> NQSVVVDFLLPTGVYLNFPVSRNANLSTIKQLLWHRAQYEPLFHMLSGPEAYVFTCINQTAEQQELEDEQRRLCDVQPFLPVLRLVAREGDRVKKLINSQISLLIGKGLHEFDSLCDPEVNDFRAKMCQFCEEAAARRQQLGWEAWLQYSFPLQLEPSAQTWGPGTLRLPNRALLVNVKFEGSEESFTFQVSTKDVPLALMACALRKKATVFRQPLVEQPEDYTLQVNGRHEYLYGSYPLCQFQYICSCLHSGLTPHLTMVHSSSILAMRDEQSNPAPQVQKPRAKPPPIPAKKPSSVSLWSLEQPFRIELIQGSKVNADERMKLVVQAGLFHGNEMLCKTVSSSEVSVCSEPVWKQRLEFDINICDLPRMARLCFALYAVIEKAKKARSTKKKSKKADCPIAWANLMLFDYKDQLKTGERCLYMWPSVPDEKGELLNPTGTVRSNPNTDSAAALLICLPEVAPHPVYYPALEKILELGRHSECVHVTEEEQLQLREILERRGSGELYEHEKDLVWKLRHEVQEHFPEALARLLLVTKWNKHEDVAQMLYLLCSWPELPVLSALELLDFSFPDCHVGSFAIKSLRKLTDDELFQYLLQLVQVLKYESYLDCELTKFLLDRALANRKIGHFLFWHLRSEMHVPSVALRFGLILEAYCRGSTHHMKVLMKQGEALSKLKALNDFVKLSSQKTPKPQTKELMHLCMRQEAYLEALSHLQSPLDPSTLLAEVCVEQCTFMDSKMKPLWIMYSNEEAGSGGSVGIIFKNGDDLRQDMLTLQMIQLMDVLWKQEGLDLRMTPYGCLPTGDRTGLIEVVLRSDTIANIQLNKSNMAATAAFNKDALLNWLKSKNPGEALDRAIEEFTLSCAGYCVATYVLGIGDRHSDNIMIRESGQLFHIDFGHFLGNFKTKFGINRERVPFILTYDFVHVIQQGKTNNSEKFER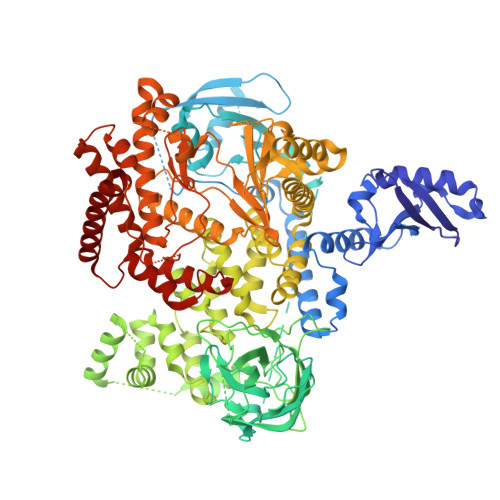FRGYCERAYTILRRHGLLFLHLFALMRAAGLPELSCSKDIQYLKDSLALGKTEEEALKHFRVKFNEALRESWKTKVNWL>[2x]MSNLKDFSQPGSGQESNFGVDFVIHYKVPAAERDEAEAGFVQLIRALTTVGLATEVRHGENESLLVFVKVASPDLFAKQVYRARLGDWLHGVRVSAPHNDIAQALQDEPVVEAERLRLIYLMITKPHNEGGAGVTPTNAKWKHVESIFPLHSHSFNKEWIKKWSSKYTLEQTDIDNIRDKFGESVAFYFAFLRSYFRFLVIPSAFGFGAWLLLGQFSYLYALLCGLWSVVFFEYWKKQEVDLAVQWGVRGVSSIQQSRPEFEWEHEAEDPITGEPVKVYPPMKRVKTQLLQIPFALACVVAAGALIVTCNSLEVFINEVYSGPGKQYLGFLPTIFLVIGTPTISGVLMGA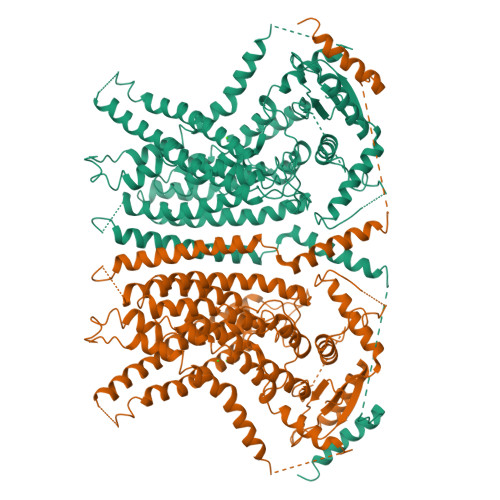AEKLNAMENYATVDAHDAALIQKQFVLNFMTSYMALFFTAFVYIPFGHILHPFLNFWRATAQTLTFSEKELPTREFQINPARISNQMFYFTVTAQIVNFATEVVVPYIKQQAFQKAKQLKSGSKVQEDHEEEAEFLQRVREECTLEEYDVSGDYREMVMQFGYVAMFSVAWPLAACCFLVNNWVELRSDALKIAISSRRPIPWRTDSIGPWLTALSFLSWLGSITSSAIVYLCSNSKNGTQGEASPLKAWGLLLSILFAEHFYLVVQLAVRFVLSKLDSPGLQKERKERFQTKKRLLQENLGQDAAEEAAAPGIEHSEKITREALEEEARQASIRGHGTPEEMFWQRQRGMQETIEIGRRMIEQQLAAGKNGKKSAPAVPSEKAS>[2x]MHH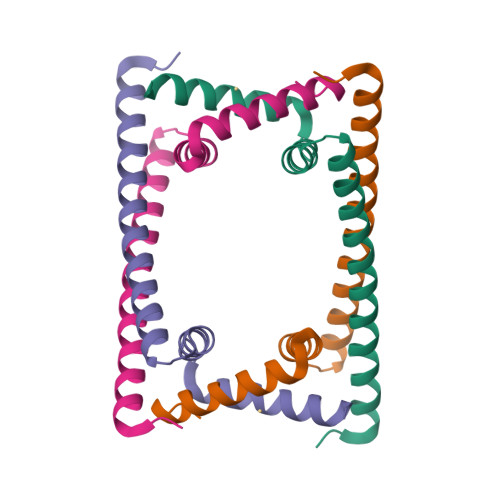HHHHHHPDLGTGSENLYFQGAMADDAIPHTDVLNSTAQGQLKSIIERVERLEVEKAEIMEQIKEVYAEAKGNGFDVKVLKKVVRIRKQDRAKRQEEDAILDLYLSAIGEI>[2x]MFIKNDHAGDRKRLEDWRIKGYDPLTPPDLLQHEFPISAKGEENIIKARDSVCDILNGKDDRLVIVIGPCSLHDPKAAYDYADRLAKISEKLSKDLLIIMRAYLEKPRTTVGWKGLINDPDMNNSFQINKGLRISREMFIKLVEKLPIAGEMLDTISPQFLSDCFSLGAIGARTTESQLHRELASGLSFPIGFKNGTDGGLQVAIDAMRAAAHEHYFLSVTKPGVTAIVGTEGNKDTFLILRGGKNGTNFDKESVQNTKKQLEKAGLTDDSQKRIMIDCSHGNSNKDFKNQPKVAKCIYDQLTEGENSLCGVMIESNINEGRQDIPKEGGREGLKYGCSVTDACIGWESTEQVLELLAEGVRNRRKALKK

3-deoxy-D-arabino-heptulosonate-7-phosphate synthase (DAHPS) is a key enzyme in the shikimate pathway for the biosynthesis of aromatic compounds. In the seven-step shikimate pathway, the first committed step involves an aldol condensation of PEP and E4P to form DAHP, catalyzed by DAHPS, which can be classified into Type I and Type II enzymes based on their sequence relationships. Plants and microbes use the shikimate pathway as the biosynthetic route to produce aromatic amino acids (AAAs), while animals rely on acquisition of essential AAAs from their foods.

To further investigate the mechanism of the D154N mutation in relieving the inhibition by L-Phe, we determined the crystal structure of Aro3 at 3.3 Å. The Aro3 crystals contain one dimer per asymmetric unit with each monomer exhibiting a canonical (β/α)8 TIM-barrel fold common to other Type Iα DAHPS enzymes. Next, we used the AutoDockTools-1.5.6 program to model the complex structures. During the simulations, L-Phe was harbored in a cavity formed by helices α3 and α4, β-sheets of β6a/β6b and their adjacent loops, and the N-terminus of the second subunit of the dimer. Strikingly, the distance between the carboxyl oxygen (OE1) of Q159 and the nitrogen (N) of L-Phe was centered around 2.8 Å in the wild-type complex, while a much longer distance (centered around 5.3 Å and 5.8 Å) was found in the Aro3D154N mutant complex. Taken together, the hydrogen bonding between L-Phe with the two key residues (Q159 and K222) of Aro3 were weakened by introducing the D154N mutation. Although the D154 of Aro3 and its counterparts of other type Iα DHAPS are located outside the inhibitor binding cavity, substitution by Asn weakened interactions between Q159/K222 and the enzyme inhibitor. The Aro3 crystal structure along with the molecular dynamics simulations analysis suggests that the D154N mutation distant from the inhibitor binding cavity may reduce the binding affinity of L-Phe. Among them, the wild-type enzyme demonstrated high binding affinity for L-Phe with a Kd of 31.4 μM. The mutant Aro3D154N exhibited weaker interactions and higher Kd value, 10-fold of the wild-type Kd.> SHNSHEVEENGSVFVKLLKASGLTLKTGENQNQLGVDQVIFQRKLFQALRKHPAYPKVIEEFVNGLESYTEDSESLRNCLLSCERLQDEEASMGTFYSKSLIKLLLGIDILQPAIIKMLFEKVPQFLFESENRDGINMARLIINQLKWLDRIVDGKDLTAQMMQLISVAPVNLQHDFITSLPEILGDSQHANVGKELGELLVQNTSLTVPILDVFSSLRLDPNFLSKIRQLVMGKLSSVRLEDFPVIVKFLLHSVTDTTSLEVIAELRENLNVQQFILPSR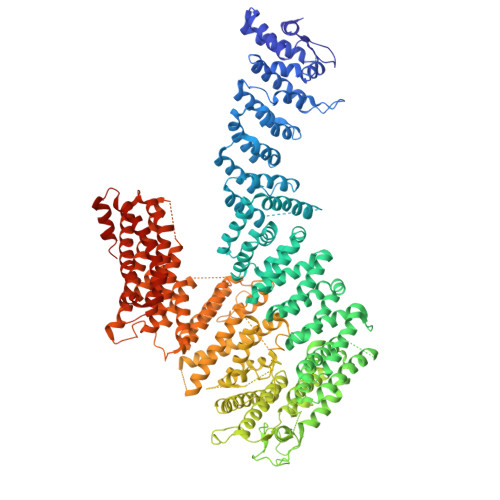IQASQSKLKSKGLASSSGNQENSDKDCIVLVFDVIKSAIRYEKTISEAWFKAIERIESAAEHKSLDVVMLLIIYSTSTQTKKGVEKLLRNKIQSDCIQEQLLDSAFSTHYLVLKDICPSILLLAQTLFHSQDQRIILFGSLLYKYAFKFFDTYCQQEVVGALVTHVCSGTEAEVDTALDVLLELIVLNASAMRLNAAFVKGILDYLENMSPQQIRKIFCILSTLAFSQQPGTSNHIQDDMHLVIRKQLSSTVFKYKLIGIIGAVTMAGIMAEDRSVPSNSSQRSANVSSEQRTQVTSLLQLVHSCTEHSPWASSLYYDEFANLIQERKLAPKTLEWVGQTIFNDFQDAFVVDFCAAPEGDFPFPVKALYGLEEYSTQDGIVINLLPLFYQECAKDASRATSQESSQRSMSSLCLASHFRLLRLCVARQHDGNLDEIDGLLDCPLFLPDLEPGEKLESMSAKDRSLMCSLTFLTFNWFREVVNAFCQQTSPEMKGKVLSRLKDLVELQGILEKYLAVIPDYVPPFASVDLDTLDMMPRKTFVSLQNYRAFFRELDIEVFSILHSGLVTKFILDTEMHTEATEVVQLGPAELLFLLEDLSQKLENMLTAPFAKRICCFKNKGRQNIGFSHLHQRSVQDIVHCVVQLLTPMCNHLENIHNFFQCLGAEHLSADDKARATAQEQHTMACCYQKLLQVLHALFAWKGFTHQSKHRLLHSALEVLSNRLKQMEQDQPLEELVSQSFSYLQNFHHSVPSFQCGLYLLRLLMALLEKSAVPNQKKEKLASLAKQLLCRAWPHGEKEKNPTFNDHLHDVLYIYLEHTDNVLKAIEEITGVGVPELVSAPKDAASSTFPTLTRHTFVIFFRVMMAELEKTVKGLQAGTAADSQQVHEEKLLYWNMAVRDFSILLNLMKVFDSYPVLHVCLKYGRRFVEAFLKQCMPLLDFSFRKHREDVLSLLQTLQLNTRLLHHLCGHSKIRQDTRLTKHVPLLKKSLELLVCRVKAMLVLNNCREAFWLGTLKNRDLQGEEIISQDPSSSESNAEDSEDG>[2x]MFNAKYVAEATGNFITVMDALKLNYNAKDQLHPLLAE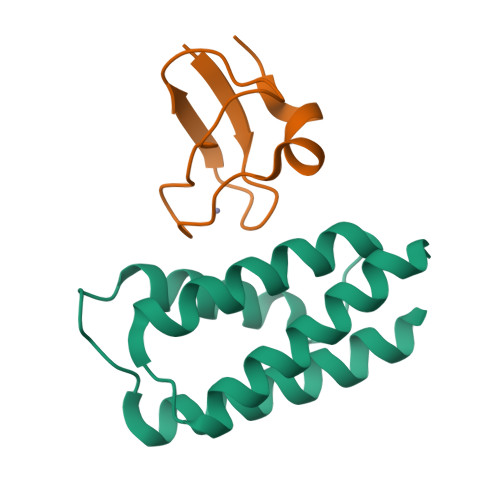LLISINRVTRDDFENRSKLIDWIVRINKLSIGDTLTETQIRELLFDLELAYKSFYALLD;>MAHHHHHHMASADVVSTWVCPICMVSNETQGEFTKDTLPTPICINCGVPADYELTKSSINCSNAIDPNANPRNQFG[2x]>QGMQTKKAFLYVFNTMSDWEYGYLIAELNSGRYFKKDLAPLKVITVGANKEMITTMGGLRIKPDISLDECTLESKDLLILPGGTTWSEEIHQPILERIGQALKIGTIVAAICGATDALANMGYLDTRKHTSNNLE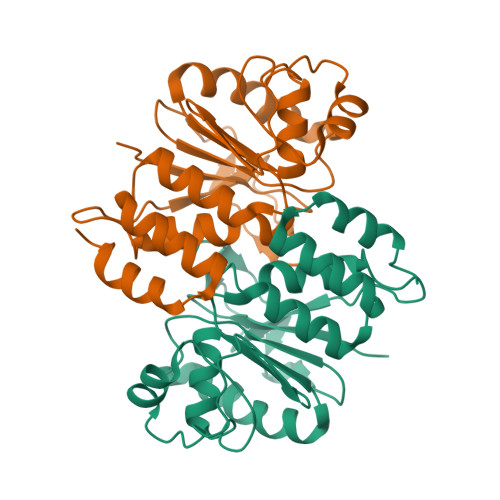YTKMVCPNYKGEKFYELGPAVSDANLVTASGIAPLEFAMEVLKKIDVFTLDALHSWYNLNKTHKPEYFFQLMNSINK[6x]Five members of the CLC family of Cl− channels and Cl−/H+ exchangers, ClC-3, ClC-4, ClC-5, ClC-6 and ClC-7, have critical roles in endosomes and lysosomes, catalyzing the exchange of two Cl− ions for one H+ ion2,10–12. We recently found that the ClC-3, ClC-4 and ClC-5 clade of endosomal CLC transporters requires the accessory β-subunit TMEM9, which we refer to as T9A or its closely related homolog TMEM9B (T9B) for proper activity in cells and animals. To resolve the mechanism by which T9A and T9B regulate the activity of ClC-3, ClC-4 and ClC-5, we determined structures of ClC-3 alone and in complex with T9A, finding that T9A occludes the Cl− ion pathway and that inhibition requires the endolysosomal signaling lipid phosphatidylinositol 3,5-bisphosphate (PtdIns(3,5)P2). Each ClC-3 protomer comprises a cytosolic N-terminal domain (NTD), a transmembrane domain (TMD) and a cytosolic domain (CD).

Analysis of cryo-EM images of ClC-3 in complex with T9A revealed four classes that can be distinguished by the densities corresponding to T9A. Despite being coexpressed with T9A, we did not observe any densities corresponding to the T9A protomers in the fourth class, possibly because of T9A dissociation during purification. To distinguish this fourth class from the structure of ClC-3 determined in the absence of T9A, we call this class ClC-3/noT9A. A weaker density is also resolved in the same position in ClC-3/noT9A, suggesting that PtdIns(3,5)P2 may bind with lower occupancy when T9A is not stably bound.

>[2x]MESEQLFHRGYYRNSYNSITSASSDEELLDGAGVIMDFQTSEDDNLLDGDTAVGTHYTMTNGGSINSSTHLLDLLDEPIPGVGTYDDFHTIDWVREKCKDRERHRRINSKKKESAWEMTKSLYDAWSGWLVVTLTGLASGALAGLIDIAADWMTDLKEGICLSALWYNHEQCCWGSNETTFEERDKCPQWKTWAELIIGQAEGPGSYIMNYIMYIFWALSFAFLAVSLVKVFAPYACGSGIPEIKTILSGFIIRGYLGKWTLMIKTITLVLAVASGLSLGKEGPLVHVACCCGNIFSYLFPKYSTNEAKKREVLSAASAAGVSVAFGAPIGGVLFSLEEVSYYFPLKTLWRSFFAALVAAFVLRSINPFGNSRLVLFYVEYHTPWYLFELFPFILLGVFGGLWGAFFIRANIAWCRRRKSTKFGKYPVLEVIIVAAITAVIAFPNPYTRLNTSELIKELFTDCGPLESSSLCDYRNDMNASKIVDDIPDRPAGIGVYSAIWQLCLALIFKIIMTVFTFGIKVPSGLFIPSMAIGAIAGRIVGIAVEQLAYYHHDWFIFKEWCEVGADCITPGLYAMVGAAACLGGVTRMTVSLVVIVFELTGGLEYIVPLMAAVMTSKWVGDAFGREGIYEAHIRLNGYPFLDAKEEFTHTTLAADVMRPRRNDPPLAVLTQDNMTVDDIENMINETSYNGFPVIMSKESQRLVGFALRRDLTIAIESARKKQEGIVGSSRVCFAQHTPSLPAESPRPLKLRSILDMSPFTVTDHTPMEIVVDIFRKLGLRQCLVTHNGRLLGIITKKDILRHMAQTANQDPASIMFN> KATMQCGENEKYDSCGSKECDKKCKYDGVEEEDDEEPNVPCLVRVCHQDCVCEEGFYRNKDDKCVSAEDCELDNMDFIYPGTRN;> IVGGQECKDGECPWQALLINEENEGFCGGTILSEFYILTAAHCLYQAKRFKVRVGDRNTEQEEGGEAVHEVEVVIKHNRFTKETYDFDIAVLRLKTPITFRMNVAPACLPERDWAESTLMTQKTGIVSGFGRTHEKGRQSTRLKMLEVPYVDRNSCKLSSSFIITQNMFCAGYDTKQEDACQGDSGGPHVTRFKDTYFVTGIVSWG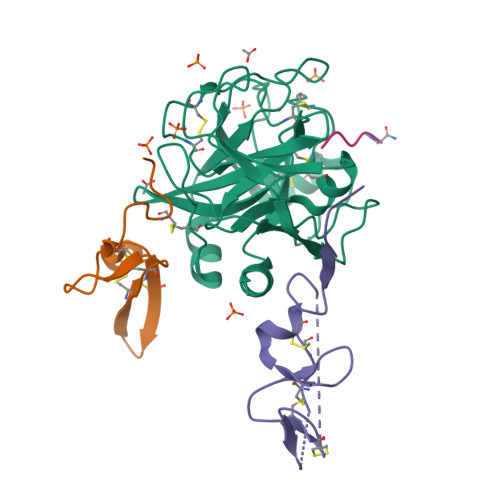EGCARKGKYGIYTKVTAFLKWIDRSMK;> DGDQCETSPCQNQGKCKDGLGEYTCTCLEGFEGKNCELFTRKLCSLDNGDCDQFCHEEQNSVVCSCARGYTLADNGKACIPTGPYPCGKQTLERRKRSVAQATSSSGEAPDSITWKPYDAADLDPTENPFDLLDFNQTQPERGDNNLTR;> YIRLP> MSRSKRDNNFYSVEIGDSTFTVLKRYQNLKPIGSGAQGIVCAAYD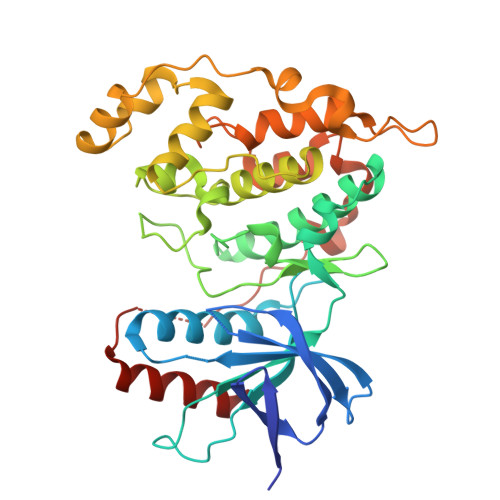AILERNVAIKKLSRPFQNQTHAKRAYRELVLMKCVNHKNIIGLLNVFTPQKSLEEFQDVYIVMELMDANLCQVIQMELDHERMSYLLYQMLCGIKHLHSAGIIHRDLKPSNIVVKSDCTLKILDFGLARTAGTSFMMTPYVVTRYYRAPEVILGMGYKENVDLWSVGCIMGEMVCHKILFPGRDYIDQWNKVIEQLGTPCPEFMKKLQPTVRTYVENRPKYAGYSFEKLFPDVLFPADSEHNKLKASQARDLLSKMLVIDASKRISVDEALQHPYINVWYDPSEAEAPPPKIPDKQLDEREHTIEEWKELIYKEVMDLE>MNLPTAQEVQGLM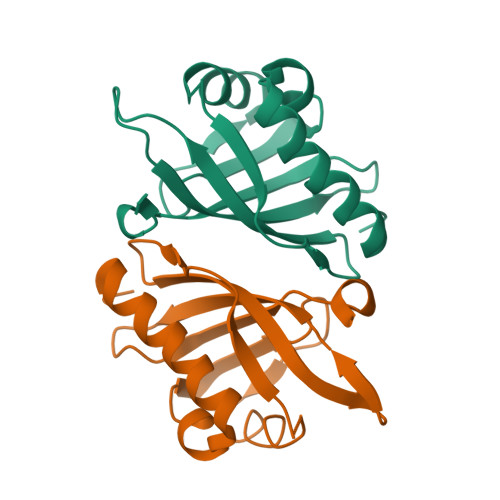ARYIELVDVGDIEAIVQMYADDATVEDPFGQPPIHGREQIAAFSRQGLGGGKVRACLTGPVRASHNGCGAMPFRVEMVWNGQPCALDVIDVMRFDEHGRIQTMQAYWSEVNLSVREPQ[2x]>MELFQYMEKYDYEQVLFCQDKESGLKAIIVIHDTTLGPALGGTRMWMYNSEEEALEDALRLARGMTYKNAAAGLNLGGGKTVIIGDPRKDKNEAMFRAFGRFIQGLNGRYITAEDVGTTVADMDIIYQETDYVTGISPEFGSSGNPSPATAYGVYRGMKAAAKEAFGSDSLEGKVVAVQGVGNVAYHLCRHLHEEGAKLIVTDINKEAVARAVEEFGAKAVDPNDIYGVECDIFAPCALGGIINDQTIPQLKAKVIAGSANNQLKEPRHGDMIHEMGIVYAPDYVINAGGVINVADELYGYNRERAMKKIEQIYDNIEKVFAIAKRDNIPTYV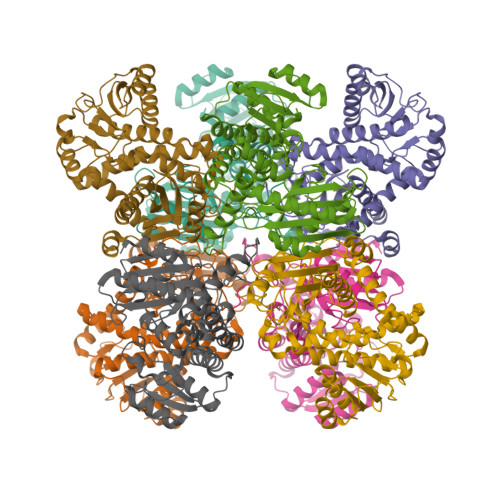AADRMAEERIETMRKARSQFLQNGHHILSRRRAR[8x]>MGSSHHHHHHSSGLVPRGSHQDPWKLSADKPDSNNYYGE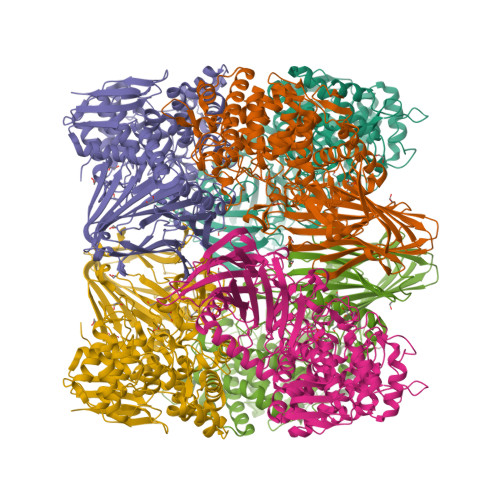TVANGMIGIISSPEPLKVKEVVLAGTYDIYKRGRVSSFIPNYNLLNMKLAFNGESVQTYNINNYKQELDMRNGAFTGSFQFKDLATVTYSYYALRHLPHCIMMVVNINTQKDTEINVENLLETPSSLNNQQNYFQNITNTHVNIPLLTSVAFTPTGRSKIAVSNTFLFDEGKKLQPEILHRMNDADMHAMSFDKKIKAGKTYSFALIGSLISSDHINDPYNEAERLTIYAALEGKSRLLNRHMQEWNSLWQSDIQVEGDPQAQQDIRSMLYHLYSFTRKSTSLSPSPMGLSGLGYNGHVFWDTEIWMFPPMLLLHPEIAKSMIEYRYQRLDAARKKAAIYGYDGAMFPWESADSGAEETPVNALTGAFEHHVTGDVAIAAWQYYLVTGDKEWLKEKGWPILKATAEFWASRVEKNDKGEYEIKNVVAADEWAENIDNNAYTNGTAIRNLQYASKCATVLGVIAPKEWTLIADKILISKMSNGVTREHDSYTDQNIKQADANLLAYPLKLITDKEQIERDLKYYQTKIPQSDTPAMTQAIFSLLYSRLEDSDQAYHWFKDAYQPNLNPPFRVISECKGGTNPYFSTGAGGVLQAVIMGFGGLDIDAAGGIKQVKSVLPKNWKKLTITGIGIEKKTFVLTH[3x]>SDTVFVRETQIPVLIERQDNVLFMLRLNAKESHTLDEVVLNFGKDVNMSDIQSVKLYYSGTEARQNYGKNFFAPVSYISSHTPGKTLAANPSYSINKSQVNNPKRKVALKANQKLFPGINYFWISLQMKPDASLLDKVAAKIAAIKVDNKEALMHTVSPENIVHRVGVGVRHAGDDGSASFRIPGLVTTNKGTLLGVYDVRYNNSADLQEHVDIGLSRSVDGGKTWEKMRLPLAFGETGDLPAAQNGVGDPSILVDTKTNTVWVVAAWTHGMGNQRAWWSSYPGMDMNHTAQLVLSKSTDDGKTWSKPINITEQVKDPSWYFLLQGPGRGITMQDGTLVFPIQFIDSTRVPNAGIMYSKDRGETWKIHNYARTNTTEAQVAEVEPGVLMLNMRDNRGGSRAISTTKDLGKTWTEHSSSRKA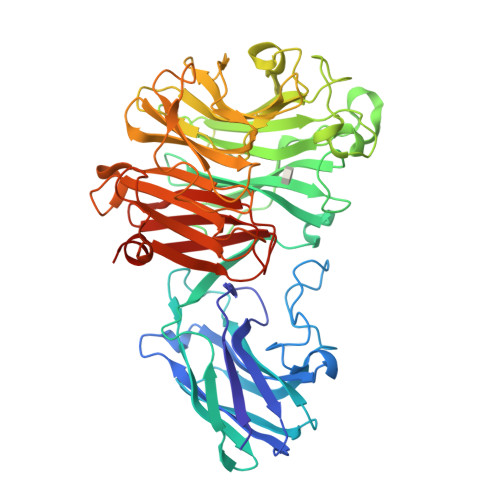LQEPVCMASLISVKAKDNVLNKDILLFSNPNTVKGRHHITIKASLDGGVTWLPEHQVMLDEGEGWGYSCLTMIDKETIGILYESSVAHMTFQAVQLRDIIKHHHH[4x]> GFPTELKPGTNQFLTTDDGVS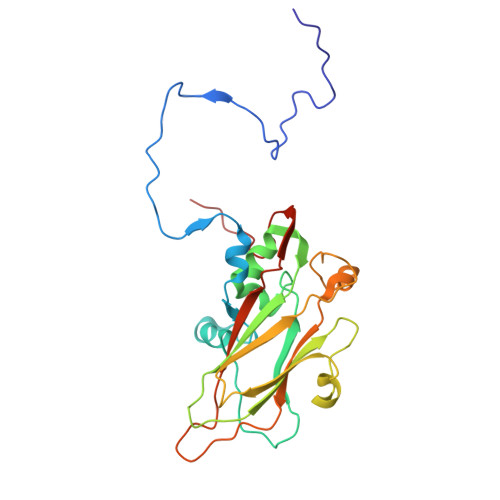APILPNFHPTPCIHIPGEVRNLLELCQVETILEVNNVPTNATSLMERLRFPVSAQAGKGELCAVFRADPGRDGPWQSTMLGQLCGYYTQWSGSLEVTFMFTGSFMATGKMLIAYTPPGGPLPKDRATAMLGTHVIWDFGLQSSVTLVIPWISNTHYRAHARDGVFDYYTTGLVSIWYQTNYVVPIGAPNTAYIIALAAAQKNFTMKLCKDTSHMLQTASIQ> GSGYREVEYWDQRYQGAADSAPYDWFGDFSSFRALLEPELRPEDRILVLGCGNSALSYELFLGGFPNVTSVDYSSVVVAAMQACYAHVPQLRWETMDVRKL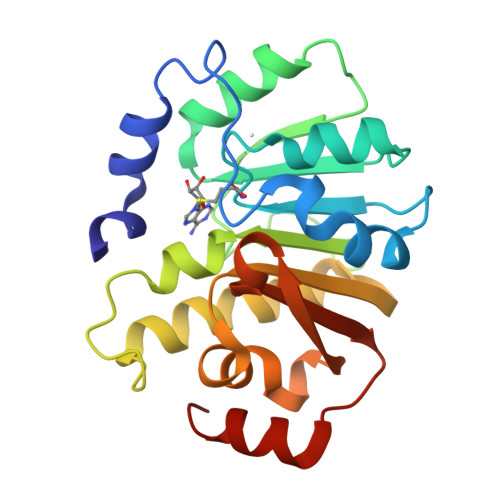DFPSASFDVVLEKGTLDALLAGERDPWTVSSEGVHTVDQVLSEVSRVLVPGGRFISMTSAAPHFRTRHYAQAYYGWSLRHATYGSGFHFHLYLMHKGGKLSVAQLALGAQILSP> ENESDKLNEEAAKNIMVGNRCEVTVGAQMARRGEVAYVGATKFKEGVWVGVKYDEPVGKNDGSVAGVRYF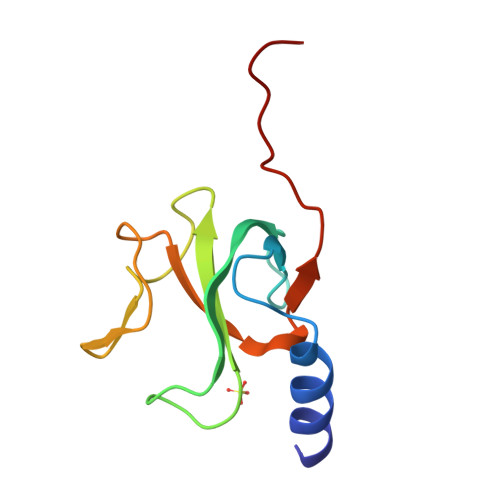DCDPKYGGFVRPVDVKVGDFPELSIDEI2-[(R)-(2-chlorophenyl)(propoxy)methyl]-1H-pyrrolo[3,2-b]pyridine-7-carboxylic 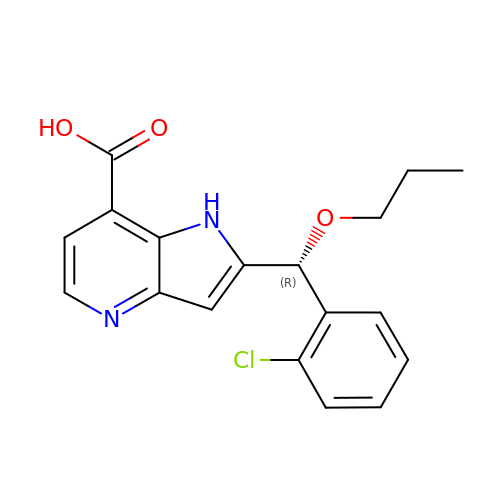acid | C18 H17 Cl N2 O3 | NXCXDWJNFKFGCO-QGZVFWFLSA-N> RSPWPGVTDKPILDCCACGTAKYRLTFYGNWSEKTHPKDYPRRANHWSAIIGGSHSKNYVLW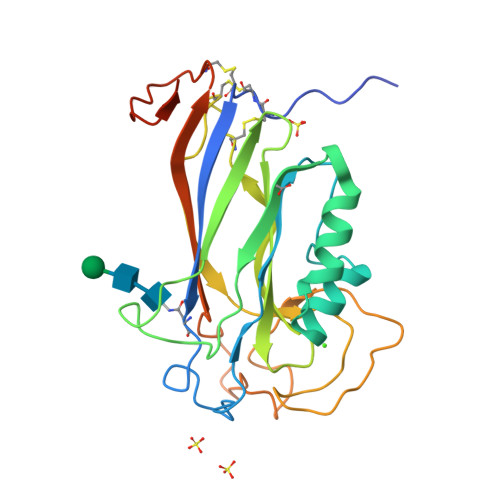EYGGYASEGVKQVAELGSPVKMEEEIRQQSDEVLTVIKAKAQWPAWQPLNVRAAPSAEFSVDRTRHLMSFLTMMGPSPDWNVGLSAEDLCTKECGWVQKVVQDLIPWDAGTDSGVTYESPNKPTIPQEKIRPLTSLDHPQSPFYDPEGGSITQVARVVIERIARKGEQCNIVPDNVDDIVADLAPEEKTGHHHHHH> MRGSHHHHHHTDPIRIELPTLIAKLNAQSKLALEQAASLCIERQHPEVTLEHYLDVLLDNPLSDVRLVLKQAGLEVDQVKQAIASTYSREQVLDTYPAFSPLLVEL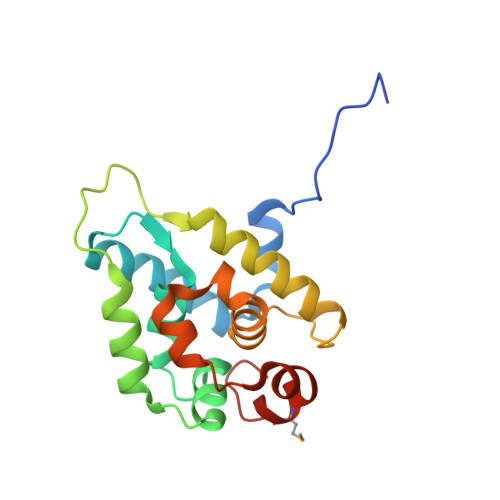LQEAWLLSSTELEQAELRSGAIFLAALTRADRYLSFKLISLFEGINRENLKKHFAMILSDSAETT> HMKELKYDVLIIGGGFAGSSAAYQLSRRGLKILLVDSKPWNRIGDKPCGDAVSKAHFDKLGMPYPKGEELENKINGIKLYSPDMQTVWTVNGEGFELNAPLYNQRVLKEAQDRGVEIWDLTTAMKPIFEDGYVKGAVLFNRRTNEELTVYSKVVVEATGYSRSFRSKLPPELPITEDLDDKDADVAYREVLLTKEDIEDHDYL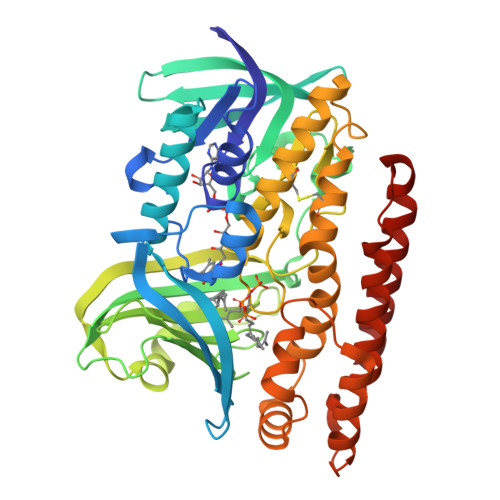RIFIDQETSPGGYWWYLPKGKNKVNVGLGIQGGMGYPSIHEYYKKYLDKYAPDVDKSKLLVKGGALVPTRRPLYTMAWNGIIVIGDSGFTVNPVHGGGKGSAMISGYCAAKAILSAFETGDFSASGLWDMNICYVNEYGAKQASLDIFRRFLQKLSNDDINYGMKKKIIKEEDLLEASEKGDLHLSVADKAMRVISGLGRPSLLFKLKAVAESMKKIKELYLNYPRSPSSLGSWRREVDNVLTEFNKSLS>GPKFPRVKNWELGSITYDTLCAQSQQDGPCTPRRCLGSLVLPRKLQTRPSPGPPPAEQLLSQARDFINQYYSSIKRSGSQAHEERLQEVEAEVASTGTYHLRESELVFGAKQAWRNAPRCVGRIQWGKLQVFDARDCSSAQEMFTYICNHIKYATNRGNLRSAITVFPQRAPGRGDFRIWNSQLVRYAGYRQQDGSVRGDPANVEITELCIQHGWTPGNGRFDVLPLLLQAPDEAPELFVLPPELVLEVPLEHPTLEWFAALGLRWYALPAVSNMLLEIGGLEFSAAPFSGWYMSTEIGTRNLCDPHRYNILEDVAVCMDLDTRTTSSLWKDKAAVEINLAVLHSFQLAKVTIVDHHAATVSFMKHLDNEQKARGGCPADWAWIVPPISGSLTPVFHQEM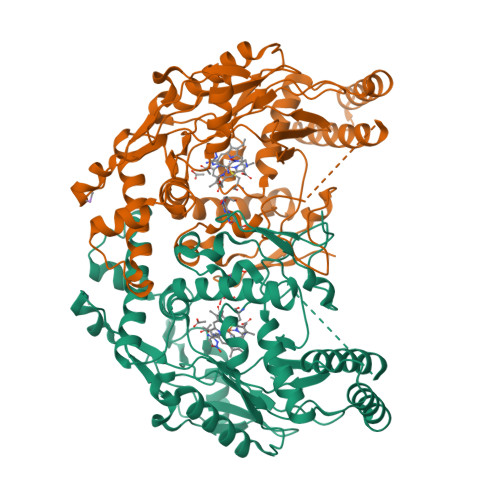VNYILSPAFRYQPDPW[2x]>MEYTFNKLTKKDVKKLKVGDIVYLNGKIYTARDEAHLKIIEMLKSNEKLPFDLNESIIYHAGPIMKKVNDSWVCVSIGPTTSARMNDVEEEFIKLTNISAIVGKGGMKKELLKTFEDYGVVYLAAPGGCAA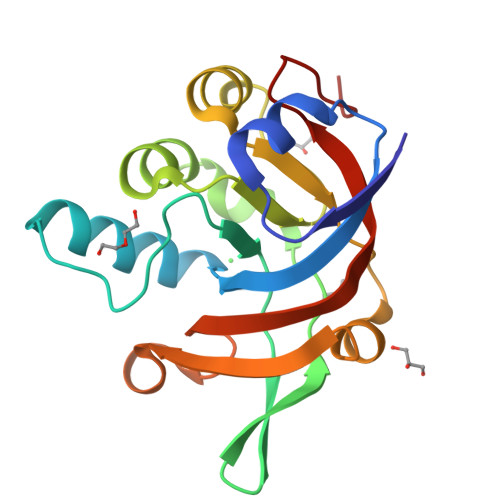LLANSVKRVDNVYFLDELGMPEAVWELEVNNFGPLIVAMDSHGNSIYE[2x]> TL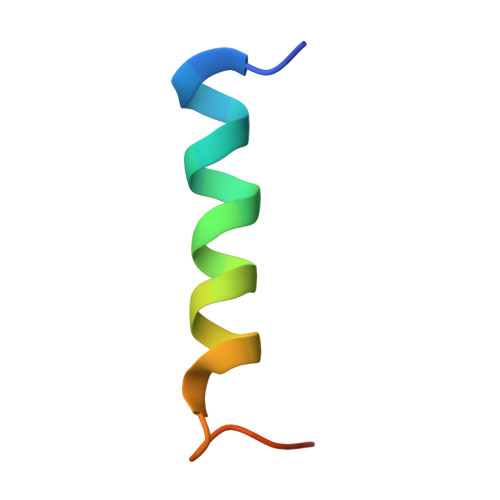DIDQSIEQLNRLILELDPTFEPIPT> GAMAPVTEKDLAEDAPWKKIQQNTFTRWCNEHLKCVNKRIGNLQTDLSDGLRLIALLEVLSQKRMYRKYHQRPTFRQMQLENVSVALEFLDRESIKLVSIDSKAIVDGNLKLILG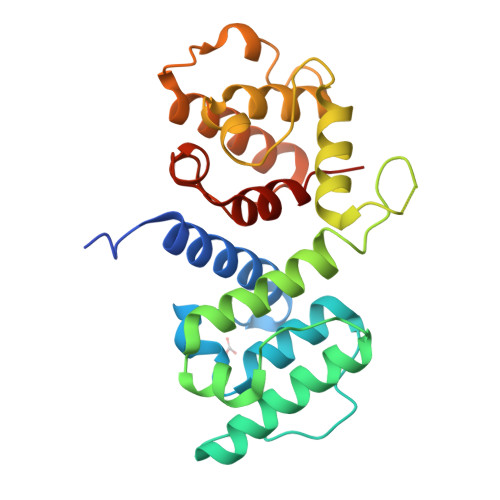LVWTLILHYSISMPVWEDEGDDDAKKQTPKQRLLGRIQNKIPYLPITNFNQNWQDGKALGALVDSCAPGLCPDWESWDPQKPVDNAREAMQQADDWLGVPQVITPEEIIHPDVDEHSVMTYLSQFPKAKL>[6x]MHHHHHHGTEKNVFNDAIVEKPNMEPAIPRPEQEKVAVSKLKNLEAKQGRKPNVLVLLVDDLGWGDPGVYGGGAAIGAPTPNIDKLANEGLRLTSMYSQPTCTSSRAALTTGRLPVRSGLVRPILTGDKVTQNPWEKEVSQGKLLSKVGYKTALIGKWHVGEAEGMLPHEVGFDYFYGLPSVQSDYTQFLVERQYADMMTNKELYTKASQLRPEGLIKGRKGGKREVAYPINSIEDISMIDQVLRDESVKFINQAVDEGKPFYLIHSFSKIHNDNYPAPKYKGASPAAMPVRDAMVEVDDITGELVALLKEKGQLENTLIIFTSDNGPNEDTWPDSGYSPWRGGKGTTWEGGVRIPGIAYWKGMISAGQVNNGLMDLTDIYMTSLRLGGVIDELPSNMYFDGIDQTAFLLADNGKSRRQVVYMWSREDFTALRWLDYKIHFKVFNTAVPRRNIDASFLLDIGTAPWVFNLNMDPKEMASTGHQYFEWGMPQATKFMKAHIATMKKYPNTDIGLGL

Here, we report the first functional characterization and the first crystal structure of a prokaryotic sulfatase, PsFucS1, belonging to sulfatase subfamily S1_13, able to release sulfate from fucoidan oligosaccharides. PsFucS1 was identified in the genome of a Pseudoalteromonas sp. isolated from sea cucumber gut. PsFucS1 (57 kDa) is Ca2+ dependent and has an unusually high optimal temperature (68 °C) and thermostability. Sulfatases represent a large family of enzymes that catalyze the hydrolytic cleavage of sulfate ester groups on carbohydrates (EC 3.1.6.-sulfuric ester hydrolases; EC 3.10.1.-sulfamidases) and are divided into four classes based on homology, crystal structures, and catalytic mechanism.

The crystals belonged to space group P212121 with six molecules in the asymmetric unit. The overall structure revealed that each PsFucS1 monomer is organized in a catalytic N-terminal domain (Asn21-Leu419) region and a C-terminal domain (Val430-Gly521) typical of the formylglycine dependent sulfatase fold. Further, the PsFucS1 displays a unique quaternary hexameric structure comprising a tight trimeric dimer complex. The structural data imply that this hexamer formation results from an uncommon interaction of each PsFucS1 monomer that is oriented perpendicular to the common dimer interface (~ 1500 Å2) that can be found in analogous sulfatases. The uncommon interaction involves interfacing (1246 Å2) through a bundle of α-helices in the N-terminal domain to form a trimeric ring structure. A single peak with an estimated apparent molecular mass of approximately 291 kDa was observed, corroborating a hexameric structure of PsFucS1 in solution, the theoretical molecular mass of which is calculated to be 345.8 kDa (and 172.4 kDa for a trimer). The active site of PsFucS1 is delineated on one side by the presence of an extended β-hairpin loop and on the other side by a bundle of three α-helices, displaying a pocket topology. Mapping electrostatic potential onto the surface of PsFucS1 highlights a positively charged pocket, perfectly suited for the recognition of a sulfate group. The active site of sulfatases normally encompasses the catalytic nucleophile formylglycine residue but the Fo-Fc difference density of the X-ray structure of PsFucS1 showed no evidence of significant maturation of the catalytic Cys111, but undoubtedly showed the unmodified cysteine. This is common in crystal structures of sulfatases that are heterologously produced in the absence of the native formylglycine-generating enzyme, since the E. coli maturation machinery is often unable to post-translationally modify the sulfatase to a substantial extent.> MNQLQQLQNPGESPPVHPFVAPLSYLLGTWRGQGEGEYPTIPSFRYGEEIRFSHSGKPVIAYTQKTWKLESGAPMHAESGYFRPRPDGSIEVVIAQSTGLVEVQKGTYNVDEQSIKLKSDLVGNASKVKEISREFELVD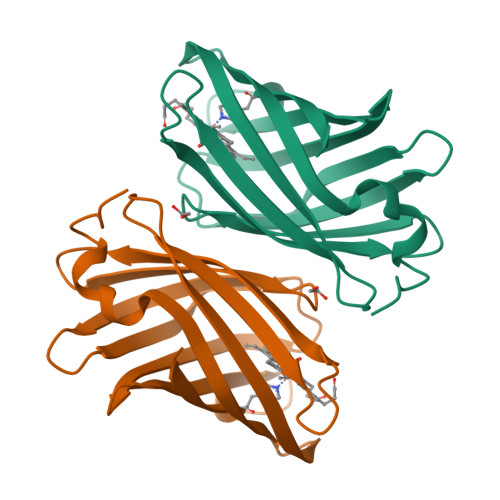GKLSYVVRMSTTTNPLQPHLKAILDKL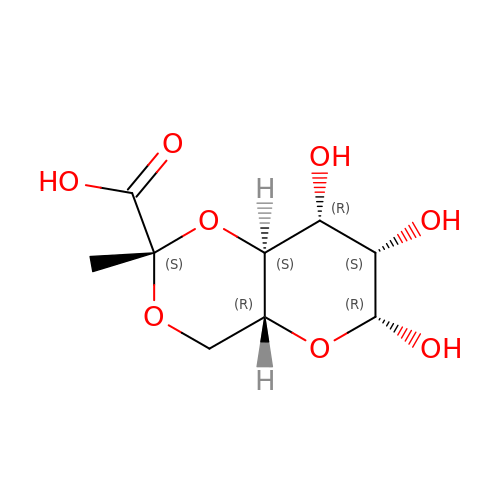(4AR,6R,7S,8R,8AS)-HEXAHYDRO-6,7,8-TRIHYDROXY-2-METHYLPYRANO[3,2-D][1,3]DIOXINE-2-CARBOXYLIC ACID | C9 H14 O8 | QVVFNJUJKXWFAU-BDIBXJNUSA-N1,5-dimethyl-6-(2-oxidanyl-6-oxidanylidene-cyclohexen-1-yl)carbonyl-3-phenyl-quinazoline-2,4-dione 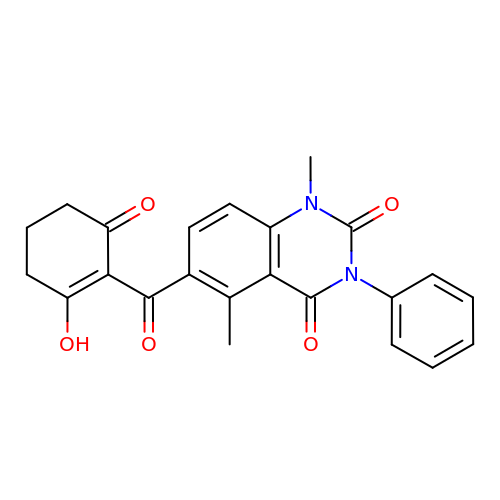| C23 H20 N2 O5 | WMCOSXYONDITDX-UHFFFAOYSA-N>[2x]MTYKIMAINAGSSSLKFQLLNMPQGALLCQGLIERIGLPEARFTLKTSAQKWQETLPIADHHEAVTLLLEALTGRGILSSLQE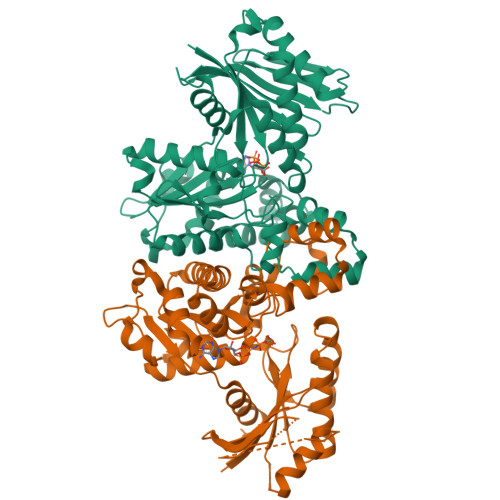IDGVGHRVAHGGERFKDAALVCDDTLREIERLAELAPLHNPVNALGIRLFRQLLPAVPAVAVFDTAFHQTLAPEAWLYPLPWRYYAELGIRRYGFHGTSHHYVSSALAEKLGVPLSALRVVSCHLGNGCSVCAIKGGQSVNTSMGFTPQSGVMMGTRSGDIDPSILPWLVEKEGKSAQQLSQLLNNESGLLGVSGVSSDYRDVEQAADAGNERAALALSLFAERIRATIGSYIMQMGGLDALIFTGGIGENSARARAAICRNLHFLGLALDDEKNQRSATFIQADNALVKVAVINTNEELMIARDVMRLALPQARELAVSA TRIAP1 (yeast Mdm35) and PRELI (yeast Ups) proteins reside within the IMS where they regulate phospholipid metabolism. Thus, lipid transfer proteins of the Ups/PRELI-family shuttle phospholipids across the IMS in a phospholipid specific manner. The partner protein TRIAP1/Mdm35 has an important role in mitochondrial import and folding of the PRELI domain as well modulating its membrane affinity. The Ups/PRELI lipid transfer proteins are widely conserved in eukaryotes and can be classified into two subfamilies by sequence similarity (Ups1/PRELID1 and Ups2/PRELID3).

In contrast, substitution of K58 by valine or threonine substantially increased the ability of PRELID1 to transfer PS, but only moderately affected its PA transfer activity. We reasoned that the mutation of the critical K58 residue in PRELID1, which promoted PS transfer, would allow phospholipid exchange and subsequent crystallisation of a PS-bound ligand. We therefore incubated PRELID1–K58V with 1:2 DOPS-DDM micelles as described by Watanabe et al. for Ups1 and PA, and following nickel purification, and SEC were able to confirm by MS that DOPS was able to displace the E. coli derived fatty acid, albeit incompletely. PRELID1–K58V incorporating DOPS formed readily crystals and diffracted to 2.98 Å. A molecule of PS was modelled into the omit map observed, and this was further refined with ligand occupancy set to 0.3 in accordance with lipidomics analysis for the PS molecule. The PS molecule docked in the observed electron density was found enclosed within the cavity of PRELID1–K58V with the serine group positioned at the bottom of the pocket and the acyl chain pointing towards the entrance of the pocket. The overall structure of the PRELI domain is largely unchanged in PRELID1–K58V mutant, showing a rmsd of 0.9 Å over the equivalent backbone atoms. The R25 side-chain, which is located near the PA phosphate of the Ups1-PA structure, is shifted towards the serine moiety in PRELID1–K58V. The smaller V58 side-chain of the mutant now allows the phosphodiester linkage to pass comfortably through and extend deeper into the cavity and the acyl chains of PS occupy the same channels as for PA. Interestingly, in the PA-bound Ups1 structure, additional space was observed beyond the phosphate deeper into the cavity and in our PS-bound PRELID1 mutant this is now occupied by the serine group from PS.

>[2x]MAHHHHHHVDDDDKMNSVGEACTDMKREYDQCFNRWFAEKFLKGDSSGDPCTDLFKRYQQCVQKAIKEKEIPIEGLEFMGHGKEKPENSS;>GSSHHHHHHSDQMVKYFLGQSVLRSSWDQVFAAFWQRYPNPYSKHVLTEDIVHREVTPDQKLLSRRLLTVTNRMPRWAERLFPANVAHSVYVLEDSIVDPQNQTMTTFTWNINHARLMVVEERSVYSVNSDNSGWTEIRREAWVSSSLFGVSRAVQEFGLARFKSNVTKTMKGFEYILAKLQGEA[2x]> SNPCAKPHGKKLATVKQIAQYYKRKAYIQLNERGSRSALKGDASQGQYDRGGKADDFKTKLC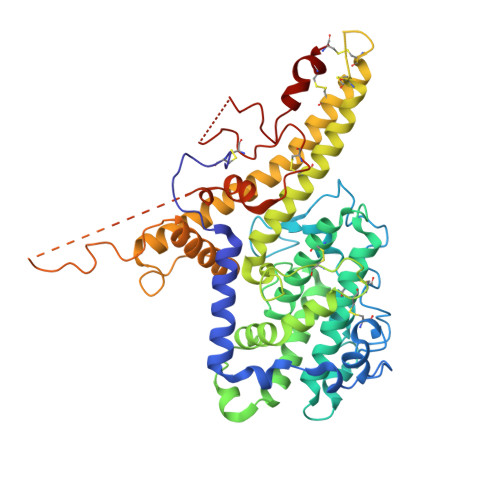EINEKHSNARSNSLNPCNGKDNNKVRFNVGTPWQSGEKIATATDVYLPPRRQHFCTSNLEYLINGGHQAILNVKNGKINHSFLGDVLLAAKYQAQHTMKDYKSKNDKEGICRAIRYSFADIGDIIKGTDLWDKDGGEIKTQNHLVTIFDKIKAQLPKDIKGKYTGTKHLELRKDWWEANRDQVWKAMQCGNDNPCSGESDHTPLHDYIPQRLRWMTEWAEWYCKEQSRLYDKLKVCEECMRKGESCTKGSGECATCKEACEEYNKEIKKWEQQWDAISYKYLMLYAKARITAINGGPGYYNTEVQEEDKPVVDFLYNLYLQNGGKKGPPPDTHRVKALIARVKRDAARNRVKRADGSSATRVTATTTITPYSTAAGYIHQEAHIGDCQKQTQFCKNKNGSDVSDTEADPTYAFRDKPHDHDTACKC Here, we show that the Ty1 retrotransposon Copia forms virus-like capsids in vivo and transfers between cells. Copia is enriched at the Drosophila neuromuscular junction (NMJ) and transported across synapses, and disrupting its expression promotes both synapse development and structural synaptic plasticity. Because Copia behaves in a viral-like manner, we used cryogenic-electron microscopy (cryo-EM) to determine the high-resolution structure of the Copia capsid and found that it is distinct from the related dArc1 capsid, with a larger internal capacity and the presence of pores similar to those used by retroviruses to carry out their reverse transcriptase activity. The capsid layer is composed of the Copiagag protein’s CA region, which contains 2 alpha-helical domains.

To enhance the resolution of the capsid region, we used local reconstruction methods to determine the structures of individual subregions of capsid known as capsomers, which are sub-assemblies that are found at the vertices or faces of the icosahedron. Because the Copia capsid adopts T = 9 geometry, there are 2 different hexameric capsomers along the faces (a hexamer with local 3-fold symmetry and a non-symmetric hexamer) and local refinement of each hexamer provided high-resolution maps (overall resolution of the non-symmetric and 3-fold symmetric hexamers are ~3.5-Å and 3.4-Å overall resolution, respectively). The high-quality maps of the locally refined capsomers allowed us to build an atomic model of the Copiagag protein with high confidence and good stereochemistry. The NTDs form central spokes at the center of each capsomer sub-assembly, while the CTD is arranged in the capsomer periphery. (D) CopiaGag non-symmetric hexamer is colored by electrostatic potential. The positively charged (blue) pore is at the center of the hexamer. In place of the spikes, the Copia capsid contains positively charged pores at the center of each hexameric or pentameric sub-assembly, similar to HIV. The positively charged pores of HIV function as gates for dNTP entry into the capsid for fueling reverse transcriptase activity. We hypothesize that the pores in the Copia capsid play a similar role.

>MDKAKRNIKPFDGEKYAIWKFRIRALLAEQDVLKVVDGLMPNEVDDSWKKAERCAKSTIIEYLSDSFLNFATSDITARQILENLDAVYERKSLASQLALRKRLLSLKLSSEMSLLSHFHIFDELISELLAAGAKIEEMDKISHLLITLPSCYDGIITAIETLSEENLTLAFVKNRLLDQEIKIKNDHNDTSKKVMNAIVHNNNNTYKNNLFKNRVTKPKKIFKGNSKYKVKCHHCGREGHIKKDCFHYKRILNNKNKENEKQVQTATSHG[6x]>MAPAAKNTSQTRRRVAVLGGNRIPFARSDGAYADASNQDMFTAALSGLVDRFGLAGERLDMVVGGAVLKHSRDFNLMRECVLGSELSPYTPAFDLQQACGTGLQAAIAAADGIAAGRYEVAAAGGVDTTSDPPIGLGDDLRRTLLKLRRSRSNVQRLKLVGTLPASLGVEIPANSEPRTGLSMGEHAAVTAKQMGIKRVDQDELAAASHRNMADAYDRGFFDDLVSPFLGLYRDDNLRPNSSVEKLATLRPVFGVKAGDATMTAGNSTPLTDGASVALLASEQWAEAHSLAPLAYLVDAETAAVDYVNGNDGLLMAPTYAVPRLLARNGLSLQDFDFYEIHEAFASV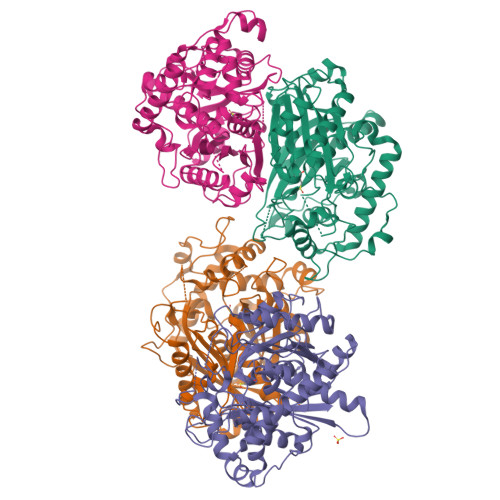VLAHLAAWESEEYCKRRLGLDAALGSIDRSKLNVNGSSLAAGHPFAATGGRILAQTAKQLAEKKAAKKGGGPLRGLISICAAGGQGVAAILEA[4x]>GSHMRSNTQTVLPFT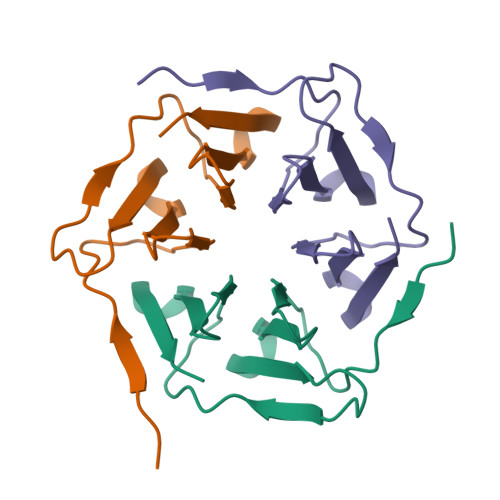GLNTPSGVAVDSAGTVYVTDRGNNRVVKLAAGSNTQTVLPFTGLNTPSGVAVDSAGTVYVTDRGNNRVVKLAAGS[3x]>[4x]SANENNLIWIDLEMTGLDPERDRIIEIATLVTDANLNIL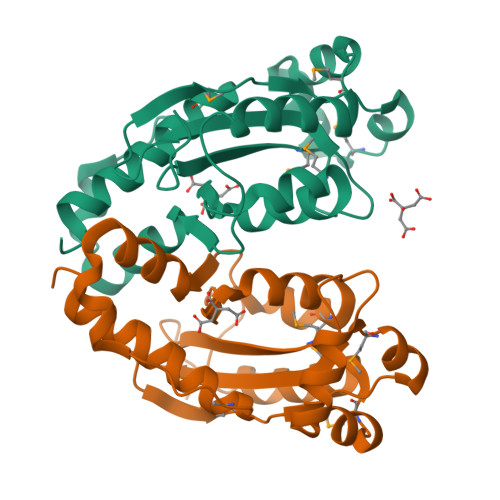AEGPTIAVHQSDEQLALMDDWNVRTHTASGLVERVKASTMGDREAELATLEFLKQWVPAGKSPICGNSIGQDRRFLFKYMPELEAYFHYRYLDVSTLKELARRWKPEILDGFTKQGTHQAMDDIRESVAELAYYREHFIKL>[2x]MADLQHIKHMRTAVRLARYALDHDETPVACIFVHTPTGQVMAYGMNDTNKSLTGVAHAEFMGIDQIKAMLGSRGVVDVFKDITLYVTVEPCIMCASALKQLDIGKVVFGCGNERFGGNGTVLSVNHDTCTLVPKNNSAAGYESIPGILRKEAIMLLRYFYVRQNERAPKPRSKSDRVLDKNTFPPMEWSKYLNEEAFIETFGDDYRTCFANKVDLSSNSVDWDLIDSHQDNIIQELEEQCKMFKFNVHKKSKV;>GPHMASMVKKVNNPLKIDYQNGIIENRLLQIRNFKDVNTPKLINVWSIRIDPRDSKKVIELIRNDFQKNDPVSLRHLKRIRKDIETSTLEVVLCSKEYICDEGEINNKLKSIWVGTKKYELSDDIE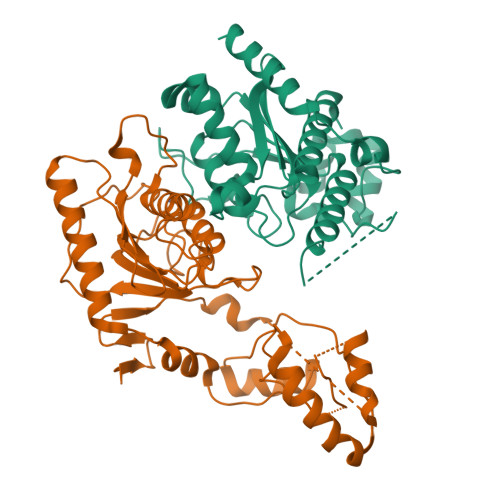VPEFAPSTKELNNAWSVKYWPLIWNGNPNDQILNDYKIDMQEVRNELSRASTLSVKMATAGKQFPMVSVFVDPSRKKDKVVAEDGRNCENSLPIDHSVMVGIRAVGERLREGVDEDANSYLCLDYDVYLTHEPCSMCSMALIHSRVRRVVFLTEMQRTGSLKLTSGDGYCMNDNKQLNSTYEAFQWIGEEYPVGQVDRDVCC[2x]> HHHHHHMIVLFVDFDYFYAQVEEVLNPSLKGKPVVVCVFSGRFEDSGAVATANYEARKFGVKAGIPIVEAKKILPNAVYLPMRKEVYQQVS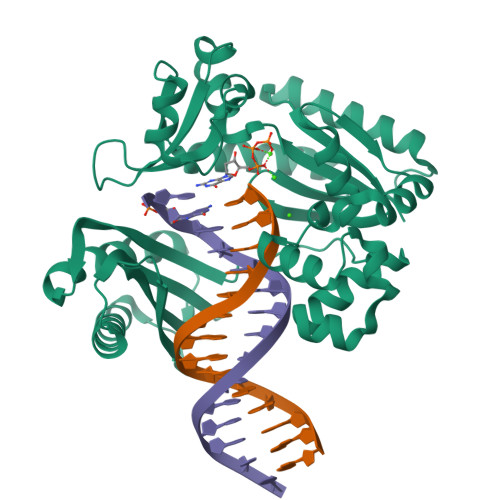SRIMNLLREYSEKIEIASIDEAYLDISDKVRDYREAYNLGLEIKNKILEKEKITVTVGISKNKVFAKIAADMAKPNGIKVIDDEEVKRLIRELDIADVPGIGNITAEKLKKLGINKLVDTLSIEFDKLKGMIGEAKAKYLISLARDEYNEPIRTRVRKSIGRIVTMKRNSRNLEEIKPYLFRAIEESYYKLDKRIPKAIHVVAVTEDLDIVSRGRTFPHGISKETAYSESVKLLQKILEEDERKIREIGVRFSKFIEAIGLDKFFDT> DTVSYDTGYDNGSRSLNDVSCSDGPNGLETRYHWSTQGQIPRFPYIGGAAAVAGWNSASCGTCWKLQYSGHTIYVLAVDHAASGFNIALDAMNALTGGQAVQLG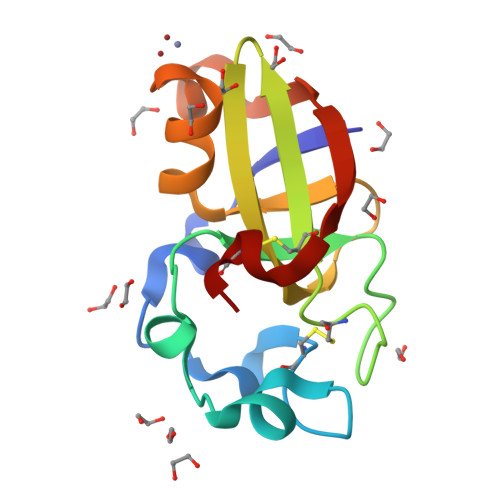RVSATATQVPVKNCGL>[2x]MSMDISDFYQTFFDEADELLADMEQHLLVLQPEAPDAEQLNAIFRAAHSIKGGAGTFGFSVLQETTHLMENLLDEARRGEMQLNTDIINLFLETKDIMQEQLDAYKQSQEPDAASFDYICQALRQLALEAKGETPSAVTRLSVVAKSEPQDEQSRSQSPRRIILSRLKAGEVDLLEEELGHLTTLTDVVKGADSLSAILPGDIAEDDITAVLCFVIEADQITFETVEVSPKISTPPVLKLAAEQAPTGRVEREKTTRSNESTSIRVAVEKVDQLINLVGELVITQSMLAQRSSELDPVNHGDLITSMGQLQRNARDLQESVMSIRMMPMEYVFSRYPRLVRDLAGKLGKQVELTLVGSSTELDKSLIERIIDPLTHLVRNSLDHGIELPEKRLAAGKNSVGNLILSAEHQGGNICIEVTDDGAGLNRERILAKAASQGLTVSENMSDDEVAMLIFAPGFSTAEQVTDVSGRGVGMDVVKRNIQKMGGHVEIQSKQGTGTTIRILLPLTLAILDGMSVRVADEVFILPLNAVMESLQPREADLHPLAGGERVLEVRGEYLPIVELWKVFNVAGAKTEATQGIVVILQSGGRRYALLVDQLIGQHQVVVKNLESNYRKVPGISAATILGDGSVALIVDVSALQAINREQRMANTAA;>[2x]MTGMTNVTKLASEPSGQEFLVFTLGDEEYGIDILKVQEIRGYDQVTRIANTPAFIKGVTNLRGVIVPIVDLRIKFSQVDVDYNDNTVVIVLNLGQRVVGIVVDGVSDVLSLTAEQIRPAPEFAVTLSTEYLTGLGALGDRMLILVNIEKLLNSEEMALLDSAASEVA;>[12x]MLKRIKIVTSLLLVLAVFGLLQLTSGGLFFNALKNDKENFTVLQTIRQQQSTLNGSWVALLQTRNTLNRAGIRYMMDQNNIGSGSTVAELMESASISLKQAEKNWADYEALPRDPRQSTAAAAEIKRNYDIYHNALAELIQLLGAGKINEFFDQPTQGYQDGFEKQYVAYMEQNDRLHDIAVSDNNASYSQAMWILVGVMIVVLAVIFAVWFGIKASLVAPMNRLIDSIRHIAGGDLVKPIEVDGSNEMGQLAESLRHMQGELMRTVGDVRNGANAIYSGASEIATGNNDLSSRTEQQAASLEETAASMEQLTATVKQNAENARQASHLALSASETAQRGGKVVDNVVQTMRDISTSSQKIADIISVIDGIAFQTNILALNAAVEAARAGEQGRGFAVVAGEVRNLAQRSAQAAREIKSLIEDSVGKVDVGSTLVESAGETMAEIVSAVTRVTDIMGEIASASDEQSRGIDQVGLAVAEMDRVTQQNAALVEESAAAAAALEEQASRLTEAVAVFRIQQQQRETSAVVKTVTPAAPRKMAVADSEENWETF

Upon ligand occupancy changes, chemoreceptors transmit signals across the inner membrane that modulate the autophosphorylation activity of a homodimeric histidine kinase CheA, which is coupled to receptor control by an adaptor protein CheW. CheA regulation requires the assembly of core-signaling units (CSUs)4,13,14 with a well-defined structure, comprising two chemoreceptor trimer-of-dimers (TOD), a single CheA dimer and two CheW monomers. Upon formation of the CSU, CheA undergoes pronounced tertiary rearrangement, increasing its basal activity nearly three orders of magnitude. CSUs further cluster into large, hexagonally packed chemosensory arrays, which place each CheA under the influence of as many as 20 receptors, giving rise to highly cooperative signaling responses.

Importantly, Q residues mimic the effects of methylated E residues on CheA activity, so a receptor with all four modification sites as glutamine (4Q) promotes high CheA activity, whereas a 4E receptor produces low kinase activity. We have now reconstituted in vitro monolayer systems using 4Q or 4E variants of the aspartate receptor signaling domain (TarCF), giving rise to TarCF4Q-CheA.P3.P4.P5-CheW and TarCF4E-CheA.P3.P4.P5-CheW monolayer arrays, which should display high and low kinase activity, respectively. For the 4Q system, we achieve an overall sub-nanometer resolution, which although anisotropic, enables the construction of an all-atom model of the E. coli CSU. To enable a detailed investigation of CSU structure and dynamics, we constructed an atomistic model of the E. coli complex, using the 8.4 Å-resolution 4Q density map to explicitly guide the modeling process. As no high-resolution structures exist of the cytoplasmic portion of E. coli Tar, we instead used a crystal structure of the E. coli Tsr TOD (PDB 1QU741), which shares a 96% sequence similarity with Tar. Models of the E. coli CheA.P3.P4 dimer and the CheA.P5-CheW dimer were generated using template-based homology modeling from crystal structures of Thermotoga maritima CheA and CheW (PDBs 4XIV17 and 4JPB42, respectively), which are sufficiently similar (75% sequence similarity for CheA.P3.P4.P5; 55% for CheW) to permit the construction of reliable models (Methods section). The resulting fits minimally altered the conformation of the initial models (backbone root-mean-squared-deviation (RMSD) = 1.8 Å) and oriented the two TODs symmetrically with a separation of 7.4 nm. The least resolved portion of the 4Q map corresponds to the CheA.P4 domains, indicating substantial conformational heterogeneity in this region of the CSU. Strikingly, the resulting fits collapsed into just two classes of CheA conformation with similar P4 CCC. We term these classes undipped and dipped to denote the relative position of P4 with respect to the rest of the CSU structure.> VGTGWYSGSPGILYHWPEVLRIQELIMYEALLVVFLIVAIGLVGLIMLQQGKGADMGASFGAGASATLFGSSGSGNFMTRMTALLATLFFIISLVLGNI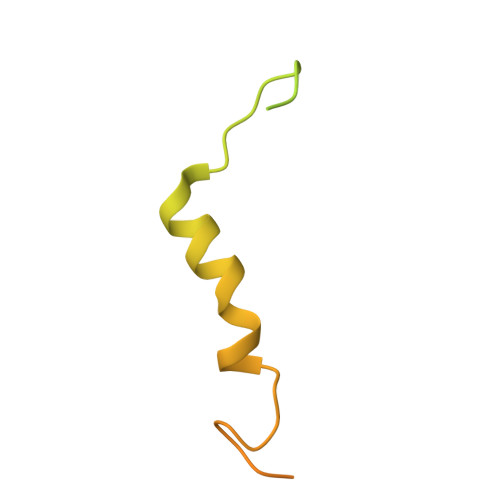NSNKTNKGSEWENLSAPAKTEQTQPAAPAKPTSDIPN> SDTGRPFVEMYSEIPEIIHMTEGRELVIPCRVTSPNITVTLKKFPLDTL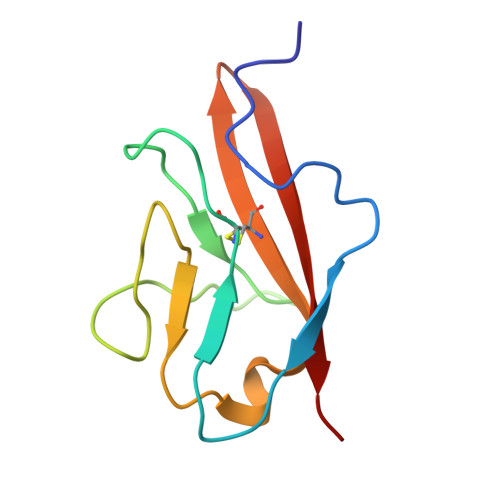IPDGKRIIWDSRKGFIISNATYKEIGLLTCEATVNGHLYKTNYLTHRQT(4-azanylcyclohexyl)methyl ~{N}-[(3~{S})-2,6-bis(oxidanylidene)piperidin-3-yl]carbamate 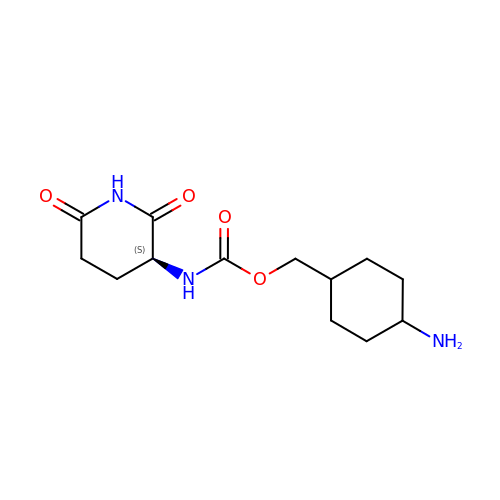| C13 H21 N3 O4 | HEPIPPZEYDEJHT-GUBZILKMSA-N> GPGSRAAQGRAFGNLGNTHYLLGNFRDAVIAHEQRLLIAKEFGDKAAERIAYSNLGNAYIFLGEFETASEYYKKTLLLARQLKDRAVEAQSCYSLGNTYTLLQDYEKAIDYHLKHLAIAQELKDRIGEGRACWSLGNAYTALGNHDQ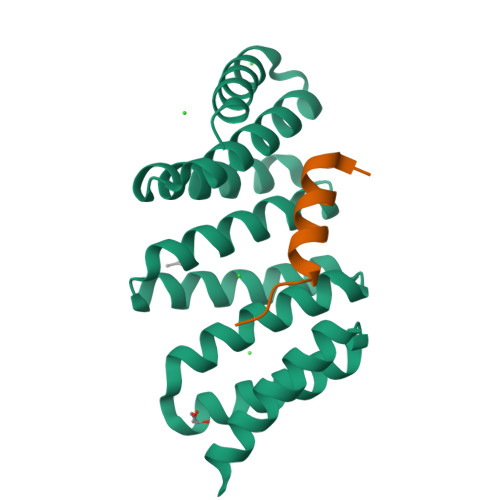AMHFAEKHLEISREVGD;> RLHFMQVDSVQRWMEDLKLMTE>MSVVISDAWRQRFGGTA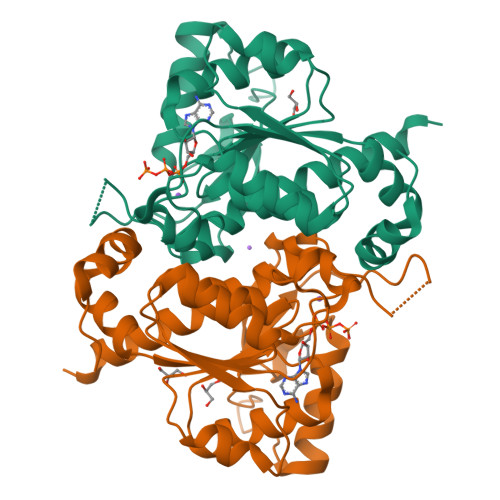RLYGEKALQLFADAHICVVGIGGVGSWAAEALARTGIGAITLIDMDDVCVTNTNRQIHALRDNVGLAKAEVMAERIRQINPECRVTVVDDFVTPDNVAQYMSVGYSYVIDAIDSVRPKAALIAYCRRNKIPLVTTGGAGGQIDPTQIQVTDLAKTIQDPLAAKLRERLKSDFGVVKNSKGKLGVDCVFSTEALVYPQSDGTVCAMKATAEGPKRMDCASGFGAATMVTATFGFVAVSHALKKMMAKAARQGLEHHHHHH[4x]> ANPCCSNPCQNRGECMSTGFDQY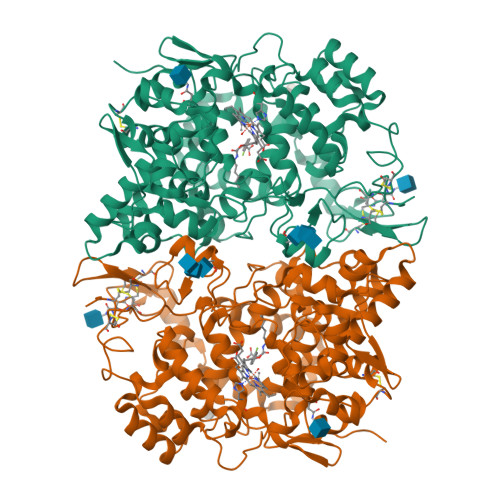KCDCTRTGFYGENCTTPEFLTRIKLLLKPTPNTVHYILTHFKGVWNIVNNIPFLRSLIMKYVLTSRSYLIDSPPTYNVHYGYKSWEAFSNLSYYTRALPPVADDCPTPMGVKGNKELPDSKEVLEKVLLRREFIPDPQGSNMMFAFFAQHFTHQFFKTDHKRGPGFTRGLGHGVDLNHIYGETLDRQHKLRLFKDGKLKYQVIGGEVYPPTVKDTQVEMIYPPHIPENLQFAVGQEVFGLVPGLMMYATIWLREHNRVCDILKQEHPEWGDEQLFQTSRLILIGETIKIVIEDYVQHLSGYHFKLKFDPELLFNQQFQYQNRIASEFNTLYHWHPLLPDTFNIEDQEYSFKQFLYNNSILLEHGLTQFVESFTRQIAGRVAGGRNVPIAVQAVAKASIDQSREMKYQSLNEYRKRFSLKPYTSFEELTGEKEMAAELKALYSDIDVMELYPALLVEKPRPDAIFGETMVELGAPFSLKGLMGNPICSPQYWKPSTFGGEVGFKIINTASIQSLICNNVKGCPFTSFNVQDPQPTKTATINASASHSRLDDINPTVLIKRRSTEL> DEALSRHFNELRTMGETLKYSEDLDFILSDNSMTTPEHRRNNMLRLCLDMMNNEDLCQYIVKYRHREVWEWCFQGTDPKQKVTSLLQCFIADKIPLLRHDKRWAMLSLENFILPLATDEVFPKKIAGSRLVKLNYQDLLRKLKFTNTCEYALYIWATYLLYTEAVYGAVPALARLISRGQLKDWDTACSLLENNIVAAPSGSDIEEYAQAFQTLAGLSREKLTNEGVLKCLIKLTNHTTVLELSADLLPSLVRSLAMSVQLHQNNIVSSISEIKTNLLILQLGLLLNIVSEATTAASTEELTNFGA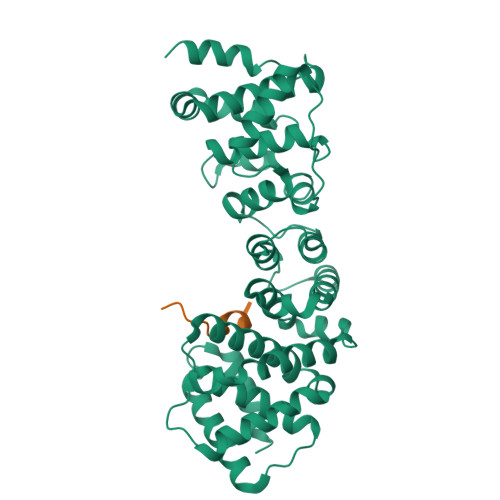VFRSVFVKKPTEMSFVLQLFLLVYAYSAGAAGVQLPPAEADFLKSELEAFATDVSSYNHNIHTRITRVLETL;> NPYNIVPQGRIVSLTNAQNRERLQLLEE> SQGHKPLEVIKIEDGVYLHTSFKNIEGYGLVDSNGLVVLDNNQAYIIDTPWSEEDTKLLLSWATDRGYQVMASISTHSHEDRTAGIKLLNSKSIPTYTSELTKKLLAREGKPVPTHYFKDDEFTLGNGLIELYYPGAGHTEDNIVAWLPKSKILFGGCLVRSHEWEGLGYVGDASISSWADSIKNIVSKKYPIQMVVPGHGKVGSSDILDHTIDLAESASNK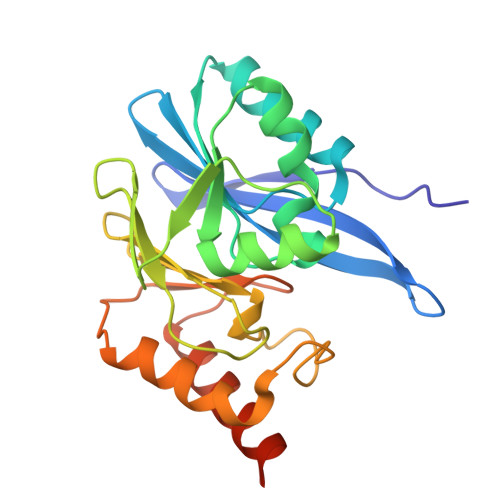LMQPTAEASAD> MSVIK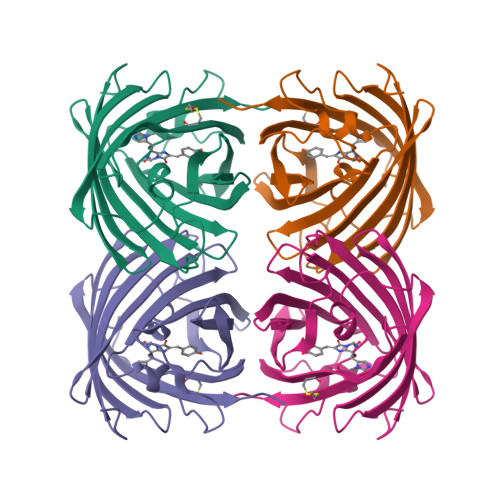SDMKIKLRMEGTVNGHKFVIEGEGEGKPYEGTQTMNLKVKEGAPLPFAYDILTTVFXNRVFAKYPKHIPDYFKQSFPEGYSWERSMTFEDGGICTARNDITLEGDCFFNEIRFDGVNFPPNGPVMQKKTLKWEPSTEKMYVRDGVLTGDINMALLLEGGGHYRCDFKTTYKAKKGVQLPDYHFVDHCIEILSHDKDYNNVKLYEHAVAHSGLPRQAKHHHHHH>GTCTCCTAG[2x];>CU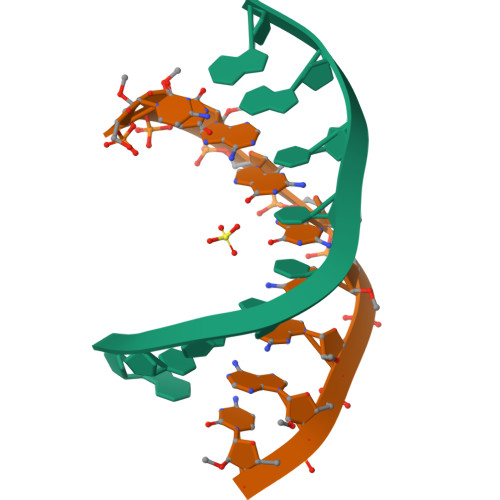AGGAGAC[2x]>[2x]LTPILFIGQGAGGQALPLLDQASIRSPLMVGCNGKPDSTPLPVDPRSLVKQGVNSNPNAALQFNAYFVDLHNPPPPFVNRLPPRPTTCGQFRASATRGRVNLEERQFFQPMAL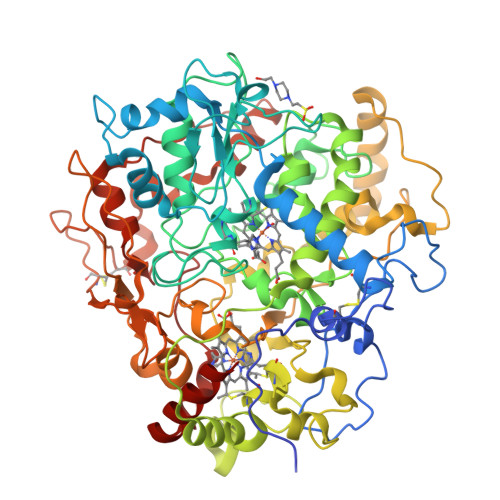ATSYHFIFLQWGYLIRPPDFEEQVSKRYGLYPAPFRNPYPLPGEDPNQTNGGSGQLPLGLIQGKDDNGRWTGLIGASCSACHDSRLGTASEASFKWGLPNSANDAGLLASDMFRTTPITALGNLLPLPWSTGRGSSDAIGLISLLPALFDMETLTLAPSLLEYVADAPHAGMTKAPAWWARAFKTRQFWDGSLSSDNVHSEMAFGVANIFRDANARRGLEDEFEDINNFLISLSPATYPKTINTALAEQGAVIYHERDLWASGANGAIPKPAGNGSCASCHGVYSPRHAADPNYLPDPRLKGVAAVVTPIETIRTDPRRMRLMADERQRRAWNSGWWAYNNLSPSWTGYPSDNIVASELRRVPRAIYNNGGPIYSPLGPNIWEEPTGYIAPPLYGAWATAPYFHNGSVPNLWGVLKPSDRPKLWKRPYTAAGIGGKNAGYDYSFASYDWQKLGWKYTAVACNNSIFTSPFLPCTHNMATIDILYSMWDNVAAQYLNLAYQSPPPITDQQIKSRMVYNSYLYGNDNGGHDFTQSLTDSERWALIEYIKTL> MKIVKHDGYNDIFNGGADGSPKPFFMSDASYHVGSFYNDNATAKRIVDVIPEEMVTAGFKMSGVKDEKEFKSLWDSYKLDSSLVDLLCWARLYGGAAMVAIIKDNRMLTSQAKPGAKLEGVRVYDRFAITVEKRVTNARSPRYGEPEIYKVSPGDNMQPYLIHHSRVFIADGERVAQQARKQNQGWGASVLNKSLIDAICDYDYCESLATQILRRKQQAVWKVKGLAEMCDDDDAQYAARLRLAQVDDNSGVGRAIGIDAETEEYDVLNSDISGVPEFLSSKM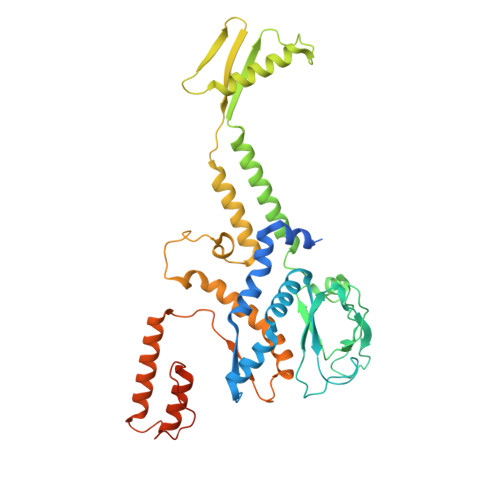DRIVSLSGIHEIIIKNKNVGGVSASQNTALETFYKLVDRKREEDYRPLLEFLLPFIVDEEEWSIEFEPLSVPSKKEESEITKNNVESVTKAITEQIIDLEEARDTLRSIAPEFKLKDGNNINIREPEETTEPEPGLGEKLEDEN> SGX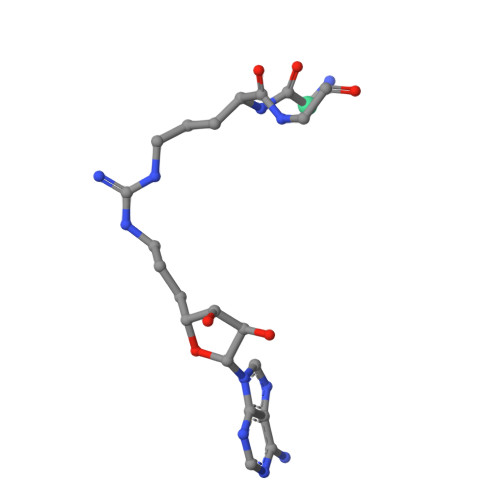GKGG>[8x]MEFTYSYLFRMISHEMKPKADQKLEQFDITNEQGHTLGYLYAHQQDGLTQNDIAKALQRTGPTVSNLLRNLERKKLIYRYVDAQDTRRKNIG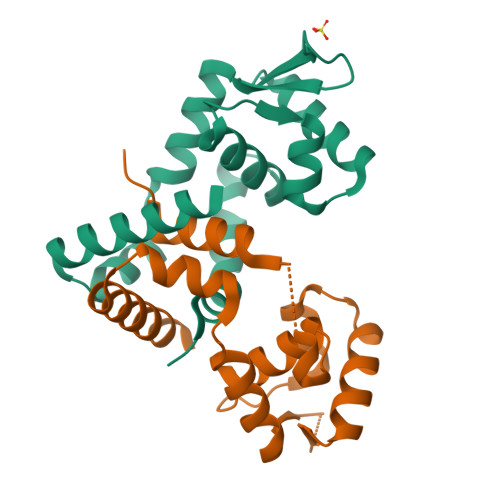LTTSGIKLVEAFTSIFDEMEQTLVSQLSEEENEQMKANLTKMLSSLQHHHHHH> VSETLVENFLSRAALVSKRSFEYKDHTSSTAQTDKNFFKWTINTRSFVQLRRKLELFTYLRFDAEITILTTVAVNGSNNNTYVGLPDLTLQAMFVPTGALTPEKQDSFHWQSGSNASVFFKISDPPARMTIPFMCINSAYSVFYDGFAGFEKTGLYGINPADTIGNLCVRIVNEHQPVGFTVTVRVYMKPKHIKAWAPRPPRTLPYMSIANA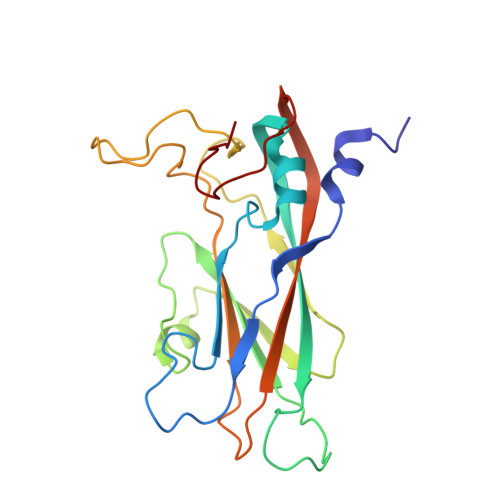NYKG>MKSSHHHHHHENLYFQSNAKEQDLDQLNTLIGIANLKKVLSVWESNKLTNTSEKFWQSVLKENTWILSQIFSNPTVLINDEAYVGGKTVKNDSGKLVDFLYANPFSKDAVLIAIKTPSTPLITPTEYRTGVYSAHKDLTGA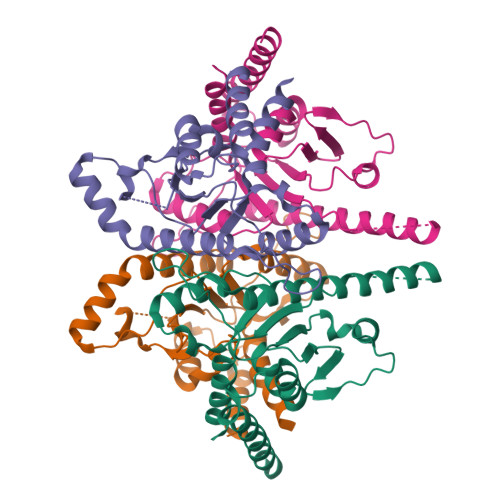VTQVLTYKTTLQREYQNIDYNNYRQGIKTDFDIITPCCVVIAGMFDTLTDTAHRHSFELYRKELKNVTVITFDELFERVKGLIKLLEG[4x]>[2x]MT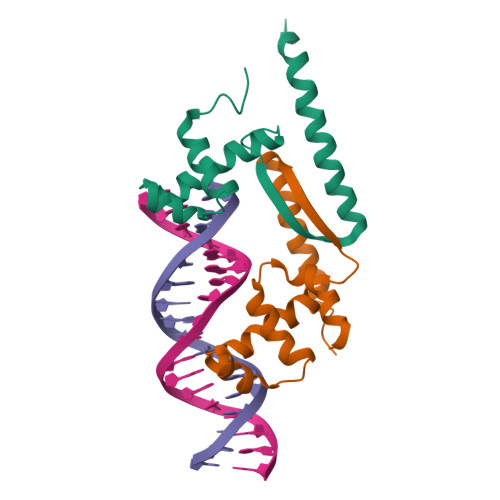AAAFDDLRPRLGRLTEETIDIAREVLVEGKSQSDVARERGLSRQRVSSMVKSVVSAANEIPREWQRVEVWLPPNLAEKVRQMEADAKADVARKNQLTDAALEHHHHHH>[5x]GQDMVSPPPPIADEPLTVNTGIYLIECYSLDDKAETFKVNAFLSLSWKDRRLAFDPVRSGVRVKTYEPEAIWIPEIRFVNVENARDADVVDISVSPDGTVQYLERFSARVLSPLDFRRYPFDSQTLHIYLIVRSVDTRNIVLAVDLEKVGKNDDVFLTGWDIESFTAVVKPANFALEDRLESKLDYQLRISRQYFSYIPNIILPM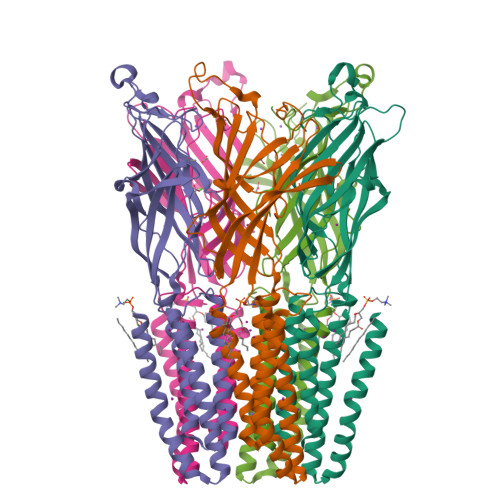LFILFISWTAFWSTSYEANVTLVVSTLIAHIAFNILVETNLPKTPYMTYTGAIIFMIYLFYFVAVIEVTVQHYLKVESQPARAASITRASRIAFPVVFLLANIILAFLFFGF> QPQFNEDTLQQRLQALIESAGENWTYAIFWQISHDFDSSTGDNTVILGWGDGYYKGEEDKEKKKNNTNTAEQEHRKRVIRELNSLISGGIGVSDESNDEEVTDTEWFFLVSMTQSFVNGVGLPGESFLNSRVIWLSGSGALTGSGCERAGQGQIYGLKTMVCIATQ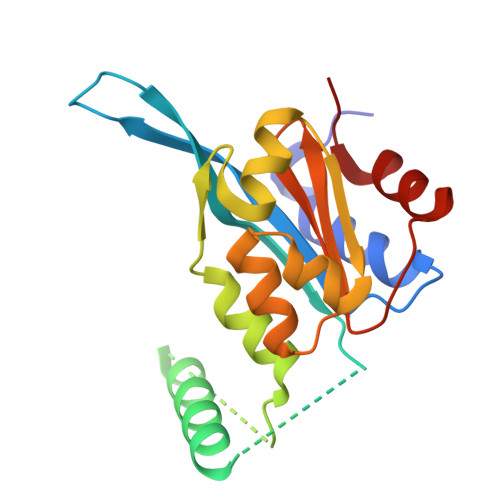NGVVELGSSEVISQSSDLMHKVNNLFNFN>MHHHHHHSTPSIVIASAARTAVGSFNGAFANTPAHELGATVISAVLERAGVAAGEVNEVILGQVLPAGEGQNPARQAAMKAGVPQEATAWGMNQLCGSGLRAVALGMQQIATGDASIIVAGGMESMSMAPHCAHLRGGVKMGDFKMIDTMIKDGLTDAFYGYHMGTTAENVAKQWQLSRDEQDAFAVASYNKAEAAQKDGRFKDEIVPFIVKGRKGDITVDADEEIRHGATLDSMAKLRPAFDKEGTVTAGNASGLNDGAAAALLMSEAEASRRGIQPLGRIVSW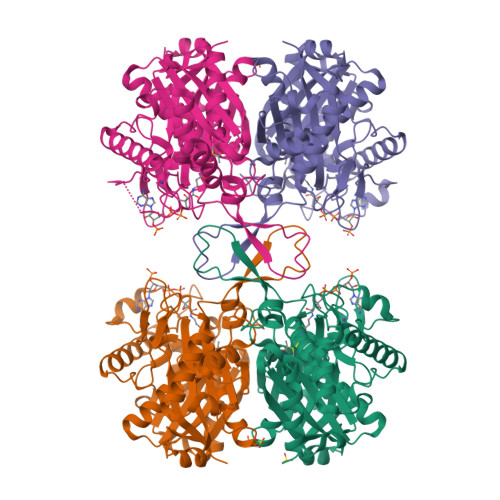ATVGVDPKVMGTGPIPASRKALERAGWKIGDLDLVEANEAFAAQACAVNKDLGWDPSIVNVNGGAIAIGHPIGASGARILNTLLFEMKRRGARKGLATLCIGGGMGVAMCIESL[4x]Breakdown is then initiated with the conversion of the C‐3 hydroxyl group to a ketone (cholest‐4‐en‐3‐one, cholestenone) by the oxidase ChoD, and further oxidation at the C‐26 “tail” region via a three‐step process involving oxidation to the hydroxyl, aldehyde, and carboxylic acid species. These sidechain‐modifying reactions are catalysed by the cytochromes P450 CYP125A1 and CYP142A1 (CYP125 and CYP142 hereafter). Comparison of the effect of complementing a CYP125 knockout in the CDC1551 strain of Mtb (which does not express the CYP142 protein), with CYP125 or CYP142 reveals that the two enzymes are functionally redundant with respect to growth on cholesterol. Here we present a series of compounds based on an ethyl 5‐(pyridin‐4‐yl)‐1H‐indole‐2‐carboxylate pharmacophore which bind strongly to both Mtb cholesterol oxidases CYP125 and CYP142.

The replacement of the cyclohexyl group with a piperazine ring, 14, showed a significant drop in affinity. The introduction of the amide group on the 2‐position of the indole 15 rescued some affinity however with both CYP125 and CYP142 these were both greater than 1 μM. In the X‐ray co‐crystal structures of compounds 14 and 15 in complex with CYP125, the pyridine coordinates directly with the heme iron, but in an orientation that is rotated almost exactly 180° around the heme vertical axis relative to compound 4.

>[2x]NGPSPNLPPGFDFTDPAIYAERLPVAEFAELRSAAPIWWNGQDPGKGGGFHDGGFWAITKLNDVKEISRHSDVFSSYENGVIPRFKNDIAREDIEVQRFVMLNMDAPHHTRLRKIISRGFTPRAVGRLHDELQERAQKIAAEAAAAGSGDFVEQVSCELPLQAIAGLLGVPQEDRGKLFHWSNEMTGNEDPEYAHIDPKASSAELIGYAMKMAEEKAKNPADDIVTQLIQADIDGEKLSDDEFGFFVVMLAVAGNETTRNSITQGMMAFAEHPDQWELYKKVRPETAADEIVRWATPVTAFQRTALRDYELSGVQIKKGQRVVMFYRSANFDEEVFQDPFTFNILRNPNPHVGFGGTGAHYCIGANLARMTINLIFNAVADHMPDLKPISAPERLRSGWLNGIKHWQVDYTGRCPVAH> EDPHLRNRPGKGHNYIDGMTQEDATCKPVTYAGACSSFDVLLEKGKFPLFQSYAHHRTLLEAVHDTIIAKADPPSCDLQSAHGNPCMKEKLVMKTHCPNDYQSA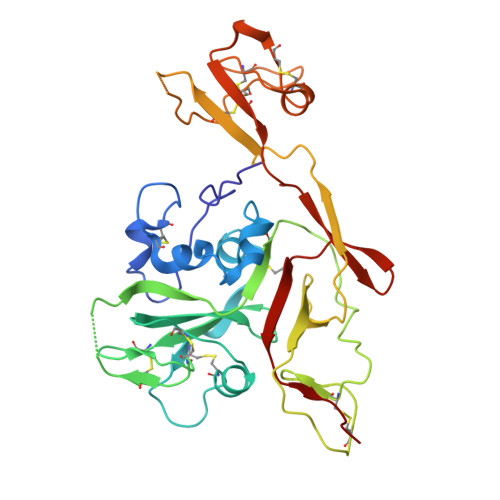HYLNNDGKMASVKCPPKYELTEDCNFCRQMTGASLKKGSYPLQDLFCQSSEDDGSKLKTKMKGVCEVGVQALKKCDGQLSTAHEVVPFAVFKNSKKVYLDKLDLKTEENLLPDSFVCFEHKGQYKGKLDSGQTKRELKSFDISQCPKIGGHGSKKCTGDAAFCSAYECTAQYANAYCSHANGSGIVQIQVSGVWKKPLCVGYERVVVKRELS>XSRRMKTQEIKNVTLEDVDFLKNLGVWVEIYHHLEKGLLQQCFNLVKKNMEALYRQSSFGWDDSEKLKEMEMEKLEYICIFEKTSKKLVGFLSFEDTVEAGLTCLYIYEIQLDEHIRGRNVGKWLLKNASILAYRRNLKYIFLTVFSANLNALN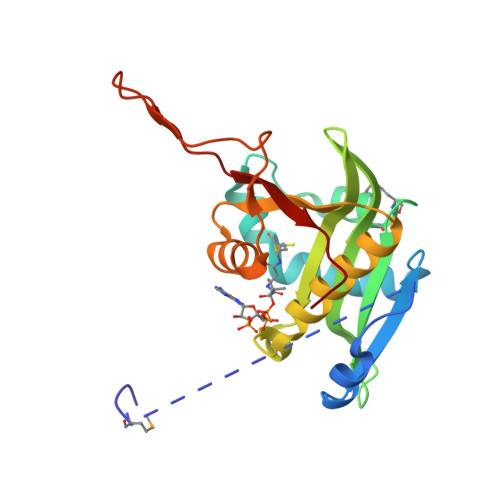FYHHFDFVPHESSPQEKKFRSGKVIHPDYYILYTKSRKDW[2x]>GPSGQEVPWLSSVRYGTVEDLLAFANHISNTAKHFYGQRPQESGILLNMVITPQNGRYQIDSDVLLIPWKLTYRNIGSDFIPRGAFGKVYLAQDIKTKKRMACKLIPVDQFKPSDVEIQACFRHENIAELYGAVLWGETVHLFMEAGEGGSVLEKLESCGPMREFEIIWVTKHVLKGLDFLHSKKVIHHDIKPSNIVFMSTKAVLVDFGLSVQMTEDVYFPKDLRGTEI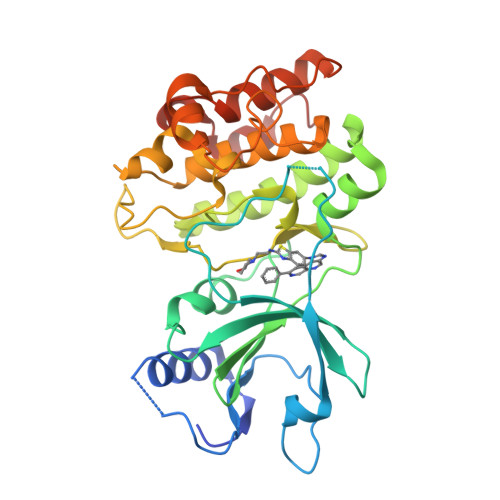YMSPEVILCRGHSTKADIYSLGATLIHMQTGTPPWVKRYPRSAYPSYLYIIHKQAPPLEDIADDCSPGMRELIEASLERNPNHRPRAADLLKHEALNPPREDQ[2x]> SSLPLNAIEPC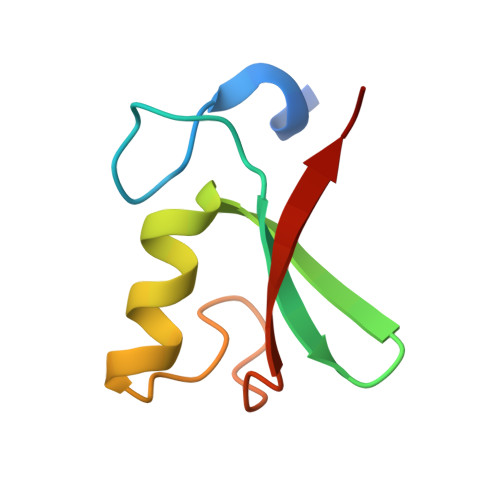VICQGRPKNGCIVHGKTGHLMACFTCAKKLKKRNKPCPVCRQPIQMIVLTYFP>GPTAVQELNRICDGMILSSILRPQMVEPSLIGDVLKTEPFTSSLEVLKDIKVSGLMRYIKQVLLGRKSYYKFGEEHADGDQNLFDYQFTGTPEEPIKGYWTTTISYRDSKPKISLTIRQEFVEGGVESQAVLATVVGRPHLQDFLLLKRKHLEYSDYPESIDLIEFGDVKVIEKTVGHGQPVVLYMASLFPIGLTKIAEQGIGCHNEKNDATLKSLLKTAILNMTPDDVSLLPRSKLDAIDHVVRNVYLRFNNSSAVSYGLHKLQSFEKILQLNGRIYETKESTLVFHHKKGVLVEDLKGLMSYKTLRVSEWREKQEPEEARVEVLEE[2x]

The two genome segments code for four viral proteins, the nucleoprotein (NP), the glycoprotein-precursor, the small matrix protein Z and the large > 200 kDa L protein which harbors the viral RNA-dependent RNA polymerase. The L protein synthesizes two distinct RNA species: (i) the antigenomic and genomic RNA as products of genome replication and (ii) the shorter capped viral mRNAs during transcription. To initiate viral transcription, the L protein presumably uses a process called cap-snatching. It is assumed that the L protein cleaves host cell mRNAs downstream of the 5'-cap structure and uses this short capped RNA as a primer for viral mRNA synthesis. Here we present the crystal structures of the two terminal domains of the CASV L protein: the cap-snatching endonuclease in the N-terminus and the 326 C-terminal residues, which, by analogy to LASV, might play a role in transcription.

Optimization of expressed fragments using bioinformatics, limited proteolysis, and thermal stability assays led to the C-terminal 326 amino acids of the CASV L protein (residues 1721–2046; residue numbering refers to the full-length L protein) with N-terminal His-tag as best candidate for structure determination. After His-tag cleavage, the purified seleno-methionine-labelled protein was successfully crystallized and the structure was solved using the single anomalous dispersion method. The protein (called CASV L-Cterm) crystallized in space group P212121 with two molecules per asymmetric unit and the structure could be refined to a resolution of 2 Å. The protein crystallized as a dimer, which is not fully symmetric. The protein monomer is U-shaped and consists of two separate domains, (i) a mainly α-helical domain (domain 1) composed of residues 1721–1793 and 1894–2046 with a long C-terminal tail and (ii) a domain (domain 2) consisting of a large β-sheet as well as one long and two short α-helices (residues 1794–1894) (blue and green respectively). The second domain is inserted into the sequence of the first one and both domains are connected by two long flexible linkers with barely any additional contacts. In the crystallized dimer the two U-shaped monomers interlock with each other to form a ring with a hole in the middle with a buried surface area of approximately 3000 Å2 between the monomers. Most importantly, the highest degree of similarity was seen between the L-Cterm domain 2 and the PB2 cap-binding domain. Domain 2 of L-Cterm also contains an aromatic residue (Y1872) at the end of the homologous long helix pointing in the same direction as the F404 in PB2. In conclusion, L-Cterm domain 2 is structurally similar to the PB2 cap-binding domain, although the typical aromatic sandwich for cap-binding is not complete.>MTPQNITDLCAEYHNTQIHTLNDKIFSYTESLAGKREMAIITFKNGATFQVEVPGSQHIDSQKKAIERMKDTLRIAYLTEAKVEKLCVWNNKT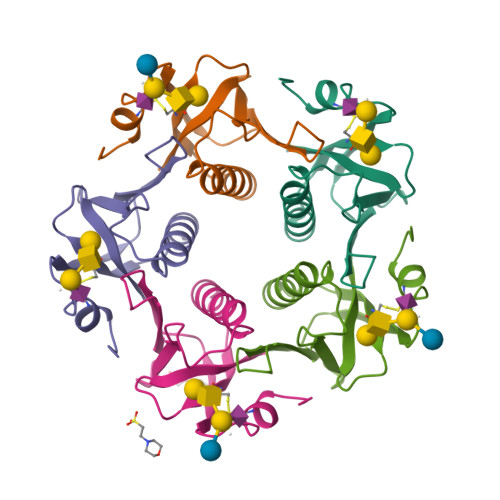PRAIAAISMAN[5x]>[6x]SNAMKMIVTEDYEEMSLVASHHVLGYITAPRRVNLAVTAGSTPKRMYEHLTAAVKGKAFYDRVHYYNFDEIPFRGQSREG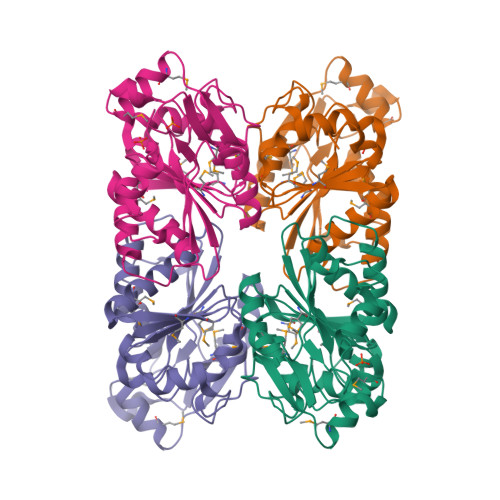VTISNLRQLFFTPAQIKEENIHKLTLDNAAQHDRQLEEAGGLDLMVLGLGADGHFCGNLPNTTRFHDQTVEVPIHGEMIALIANSEMGGDISAVPNSYVTMGPRSVMAAKNLLLIVSGAAKAHALKQVVEGPVSVQVPASVLKLHPSLVIIADKAAAAELQQ>RSYSNRTLPDTVDWREKGCVTEVKYQGSCGACWAFSAVGALEGQLKLKTGKLISLSAQNLVDCSNEEKYGNKGCGGGYMTEAFQYIIDNGGIEADASYPYKAMDEKCHYNSKNRAATCSRYIQLPFGDEDALKEAVATKGPVSVGIDASHSSFF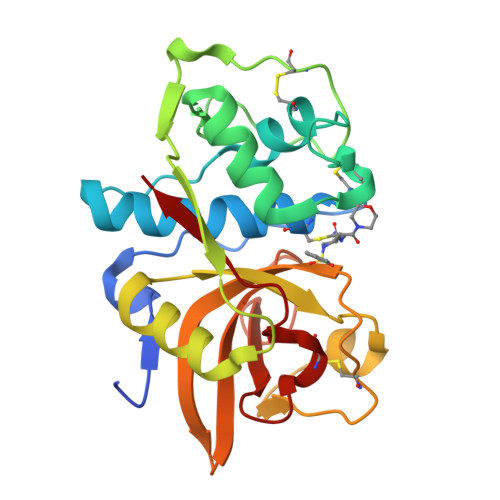FYKSGVYDDPSCTGNVNHGVLVVGYGTLDGKDYWLVKNSWGLNFGDQGYIRMARNNKNHCGIASYCSYPEI[8x]>[2x]ENLYFQGSHVYWDLDIQTNAVIKHRGPSEVLPPHPEVELLRSQLILKLRQHYRELCQQREGIEPPRESFNRWMLERKVVDKGSDPLLPSNCEPVVSPSMFREIMNDIPIRLSRIKFREEAKRLLFKYAEAARRLIESRSASPDSRKVVKWNVEDTFSWLRKDHSASKEDYMDRLEHLRRQCGPHVSAAAKDSVEGICSKIYHISLEYVKRIREKHLAILKENNISEEVEAPEVEPRLVYCYPVRLAVSAPPMPSVEMHMENNVVCIRYKGEMVKVSRNYFSKLWLLYRYSCIDDSAFERFLPRVWCLLRRYQMMFGVGLYEGTGLQGSLPVHVFEALHRLFGVSFECFASPLNCYFRQYCSAFPDTDGYFGSRGPCLDFAPLSGSFEANPPFCEELMD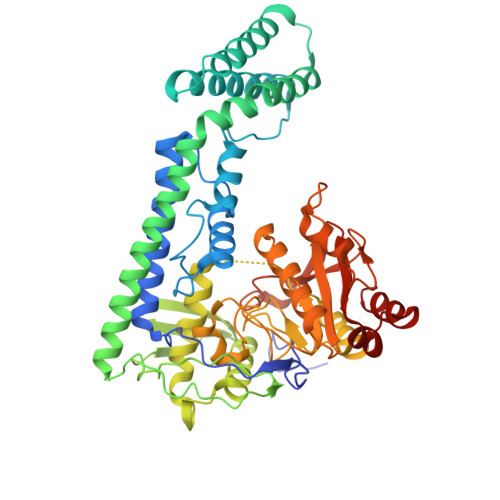AMVSHFERLLESSPEPLSFIVFIPEWREPPTPALTRMEQSRFKRHQLILPAFEHEYRSGSQHICKKEEMHYKAVHNTAVLFLQNDPGFAKWAPTPERLQELSAAYRQSGR> MRGSHHHHHHGRSLNPLSTPQFDSTDETPASYNLAVRRAAPAVVNVYNRGLNTNSHNQLEIRTLGSGVIMDQRGYIITNKHVINDADQIIVALQDGRVFEALLVGSDSLTDLAVLKINATGGLPTIPINARRVPHIGDV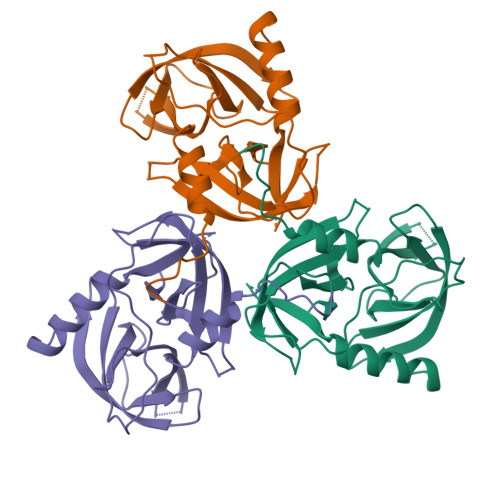VLAIGNPANLGQTITQGIISATGRIGLNPTGRQNFLQTDASINPGNSGGALVNSLGELMGINTLSFDKSNDGETPEGIGFAIPFQLATKIMDKLIRDGRVIR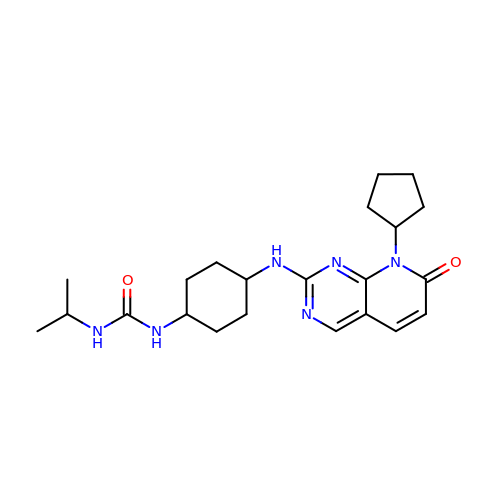1-{trans-4-[(8-cyclopentyl-7-oxo-7,8-dihydropyrido[2,3-d]pyrimidin-2-yl)amino]cyclohexyl}-3-propan-2-ylurea | C22 H32 N6 O2 | QJPUIIKZKMYPSK-QAQDUYKDSA-N> GSHMADSSSSSFFPDFGLLLYLEELNKEELNTFKLFLKETMEPEHGLTPWNEVKKA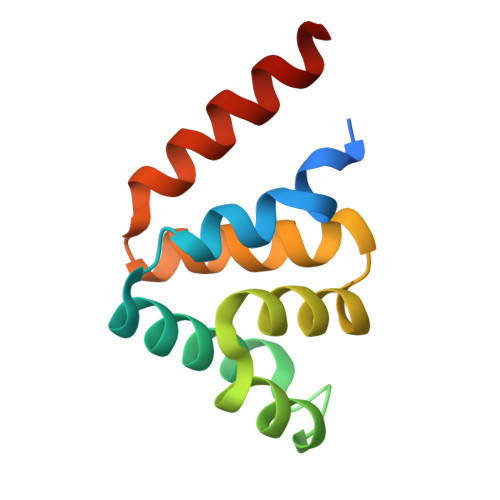RREDLANLMKKYYPGEKAWSVSLKIFGKMNRKDLCERAKEEINWSAQLE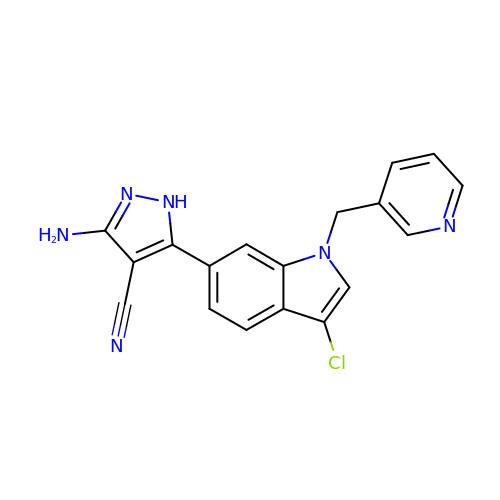3-azanyl-5-[3-chloranyl-1-(pyridin-3-ylmethyl)indol-6-yl]-1~{H}-pyrazole-4-carbonitrile | C18 H13 Cl N6 | AJLPROLDTQRMOM-UHFFFAOYSA-N> DPGTIVHNFSRTEPRTEPAGGSHSGSSSKLQALFAHPLYNVPEEPPLLGAEDSLLASQEALRYYRRKVARWNRRHKMYREQMNLTSLDPPLQLRLEASWVQFHLGINRHGLYSRSSPVVSKLLQDMRHFPTISADYSQD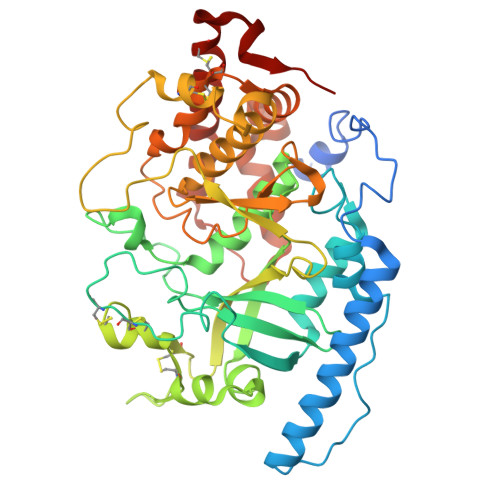EKALLGACDCTQIVKPSGVHLKLVLRFSDFGKAMFKPMRQQRDEETPVDFFYFIDFQRHNAEIAAFHLDRILDFRRVPPTVGRIVNVTKEILEVTKNEILQSVFFVSPASNVCFFAKCPYMCKTEYAVCGKPHLLEGSLSAFLPSLNLAPRLSVPNPWIRSYTLAGKEEWEVNPLYCDTVKQIYPYNNSQRLLNVIDMAIFDFLIGNMDRHHYEMFTKFGDDGFLIHLDNARGFGRHSHDEISILSPLSQCCMIKKKTLLHLQLLAQADYRLSDVMRESLLEDQLSPVLTEPHLLALDRRLQTILRTVEGCIVAHGQQSVIVDGPVEQ>MSFPYFISPEQAMRERSELARKGIARAKSVVALAYAGGVLFVAENPSRSLQKISELYDRVGFAAAGKFNEFDNLRRGGIQFADTRGYAYDRRDVTGRQLANVYAQTLGTIFTEQAKPYEVELCVAEVAHYGETKRPELYRITYDGSIADEPHFVVMGGTTEPIANALKESYAENASLTDALRIAVAALRAGSADTSGGDQPTLGVASLEVAVLDANRPRRAFRRITGSALQALLVDQESPQSDGESSG[14x];>XTIVALKYPGGVVMAGDRRSTQGNMISGRDVRKVYITDDYTATGIAGTAAVAVEF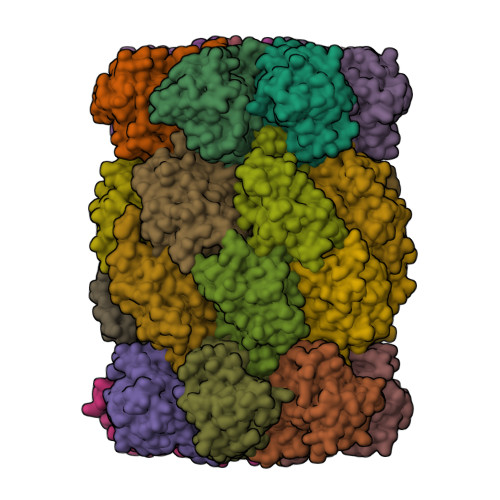ARLYAVELEHYEKLEGVPLTFAGKINRLAIMVRGNLAAAMQGLLALPLLAGYDIHASDPQSAGRIVSFDAAGGWNIEEEGYQAVGSGSLFAKSSMKKLYSQVTDGDSGLRVAVEALYDAADDDSATGGPDLVRGIFPTAVIIDADGAVDVPESRIAELARAIIESRSGADTFGSDGGEKHHHHHH[14x]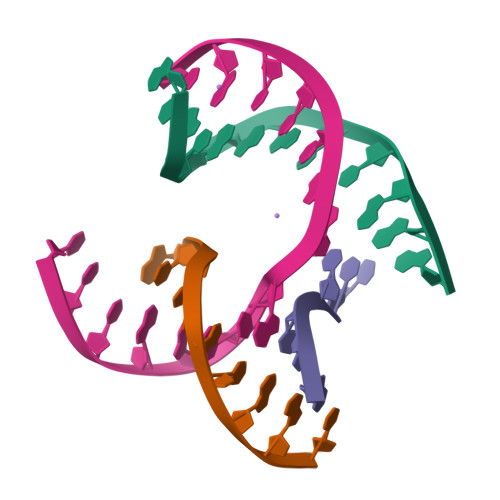> GAGCAGACCAGA;> CGACACTCA;> TCTTCG;> TCTGAGTGGGTCTGC>MAFTNYSSLNRAQLTFEYLHTNSTTHEFLFGALAELVDNARDADATRIDIYAERREDLRGGFMLCFLDDGAGMDPSDAASVIQFGKSAKRTPESTQIGQYGNGLKSGSMRIGKDFILFTKKEDTMTCLFLSRTFHEEEGIDEVIVPLPTWNARTREPVTDNVEKFAIETELIYKYSPFRTEEEVMTQFMKIPGDSGTLVIIFNLKLMDNGEPELDIISNPRDIQMAETSPEGTKPERRSFRAYAAVLYIDPRMRIFIHGHKVQTKRLSCCLYKPRMYKYTSSRFKTRAEQEVKKAEHVARIAEEKAREAESKARTLEVRLGGDLTRDSRVMLRQVQNRAITLRREADVKKRIKEAKQRALKEPKELNFVFGVNIEHRDLDGMFIYNCSRLIKMYEKVGPQLEGGMACGGVVGVVDVPYLVLEPTHNKQDFADAKEYRHLLRAMGEHLAQYWKDIAIAQRGIIKFWDEFGYLSANWNQPPSSELRYKRRRAMEIPTTIQCDLCLKWRTLPFQLSSVEKDYPDTWVCSMNPDPEQDRCEASEQKQKVPLGTFRKDMKTQEEKQKQLTEKIRQQQEKLEALQKTTPIRSQADLKKLPLEVTTRPST[2x]

The Microrchidia (MORC) family of chromatin-remodelling ATPases is pivotal in forming higher-order chromatin structures that suppress transcription. All MORCs share three features: an N-terminal gyrase, heat shock protein 90, histidine kinase and MutL (GHKL) ATPase domain, a central CW-type zinc finger (CW) domain, and a divergent C-terminal domain (CTD) with predicted coiled coils (CCs). MORC2 possesses multiple DNA-binding sites that undergo structural rearrangement upon DNA binding. Importantly, MORC2 mediates chromatin remodelling via ATP hydrolysis-dependent DNA compaction in vitro, regulated by the phosphorylation state of its CTD.

We determined the structures of MORC2PD and MORC2 ATPase domain with (MORC2PD-DNA, MORC21-603-DNA) and without DNA (MORC2PD, MORC21-603), in presence of AMP-PNP, at overall resolutions of 1.9, 2.5, 2.4 and 3.2 Å, respectively, using cryoEM. We performed electrophoretic mobility shift assay (EMSA) with MORC2WT and MORC21-603 in the presence of IRDye-700 labelled 10, 14, 19, 24, 29, 34, 39, 44, 60 and 90 bp double-stranded (dsDNA). Both constructs of MORC2 bind to dsDNA longer than 29 bp. Interestingly, almost all CC1 was missing in the DNA-bound cryoEM structures indicating high flexibility of this region upon DNA binding. Upon overlaying these models, we observed no conformational changes within the ATPase domain. In MORC21-603, we observed a significant increase in deuterium uptake in the ATP lid upon DNA binding (peptides 81 to 109), indicating an increased flexibility in the ATP lid region. The presence of DNA with MORC1-603 also reduced deuterium uptake in CC1 and nearby regions, transducer-like and CW. This suggests CC1 and nearby regions form a high-affinity DNA binding site, somewhat consistent with previous mutagenesis of the CC1 loop (point mutation of R326, R329 and R333) that prevented DNA binding. The observed flexibility of CC1 inferred from its absence in the DNA-bound MORC2 cryoEM structures and crosslinking mass spectrometry, suggests that CC1 may aid in binding and compacting DNA.>[12x]ATPHINAEMGDFADVVLMPGDPLAAKYIAETFLEDAREVNNVRGML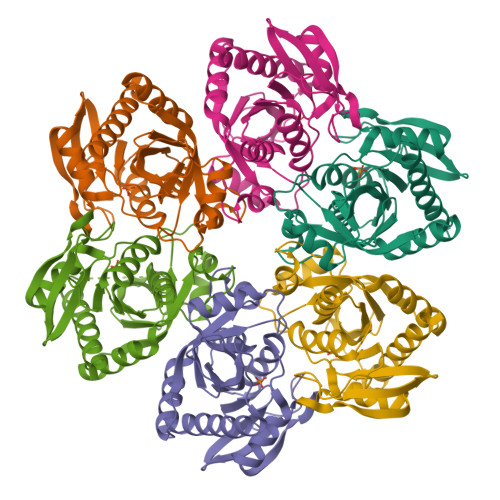GFTGTYKGRKISVMGHGMGIPSCSIYTKELITDFGVKKIIRVGSCGAVLPHVKLRDVVIGMGACTDSKVNRIRFKDHDFAAIADFDMVRNAVDAAKALGIDARVGNLFSADLFYSPDGEMFDVMEKYGILGVEMEAAGIYGVAAEFGAKALTICTVSDHIRTHEQTTAAERQTTFNDMIKIALESVLLGDK> GPHMATGQDRVVALVDMDCFFVQVEQRQNPHLRNKPCAVVAYKSWKGGGIIAVSYEARAFGVTRSMWADDAKKLCPDLLLAQVRESRGKANLTKYREASVEVMEIMSRFAVIERASIDEAYVDLTSAVQERLQKLQGQPISA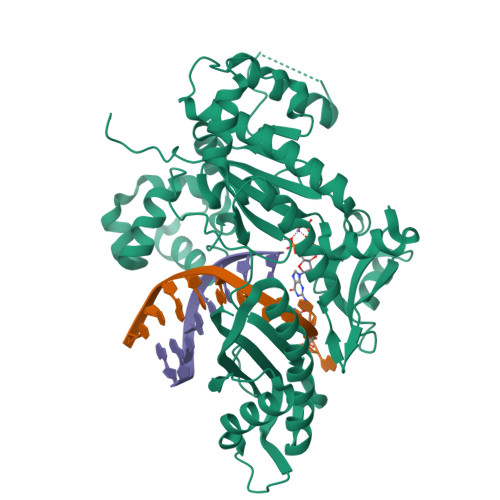DLLPSTYIEGLPQGPTTAEETVQKEGMRKQGLFQWLDSLQIDNLTSPDLQLTVGAVIVEEMRAAIERETGFQCSAGISHNKVLAKLACGLNKPNRQTLVSHGSVPQLFSQMPIRKIRSLGGKLGASVIEILGIEYMGELTQFTESQLQSHFGEKNGSWLYAMCRGIEHDPVKPRQLPKTIGCSKNFPGKTALATREQVQWWLLQLAQELEERLTKDRNDNDRVATQLVVSIRVQGDKRLSSLRRCCALTRYDAHKMSHDAFTVIKNCNTSGIQTEWSPPLTMLFLCATKFSAS> SQIPASEQETLVRPKPLLLKLLKSVGAQKDTYTMKEVLFYLGQYIMTKR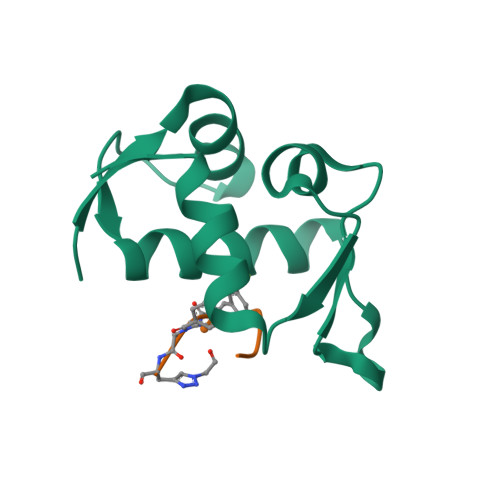LYDEKQQHIVYCSNDLLGDLFGVPSFSVKEHRKIYTMIYRNLVVVNQQESSDSGTSVSEN3-(pyridin-4-yl)benzoic acid | C12 H9 N 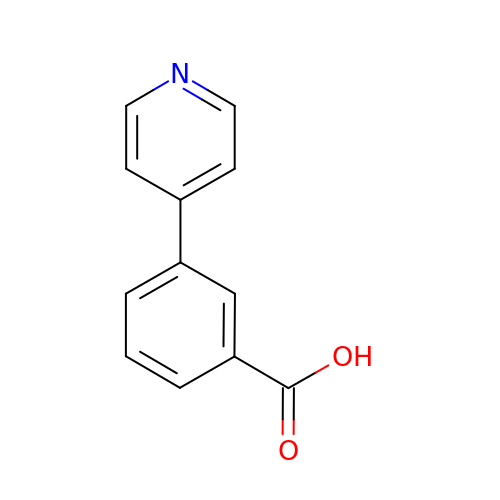O2 | IYGIZNZSONLPSI-UHFFFAOYSA-N> GELSAYTIVVGTVLTGFGFTTPLGLALIGFGTLIPVLFPAQDQSNTWSDFITQTKNIIKKEIASTYISNANKILNRSFNVISTYHNHLKTWENNPNPQNTQDVRTQIQLVHYHFQNVIPELVNSCPPNPSDCDYYNILVLSSYAQAANLHLTVLNQAVKFEAYLKNNRQFDYLEPLPTAIDYYPVLTKAIEDYTNYCVTTYKKGLNLIKTTPDSNLDGNINWNTYNTYRTKMTTAVLDLVALFPNYDVGKYPIGVQSELTREIYQVLNFEESPYKYYDFQYQEDSLTRRPHLFTWLDSLNFYEKAQTTPNNFFTSHYNMFHYTLDNISQKSSVFGNHNVTDKLKSLGLATNIYIFLLNVISLDNKYLNDYNNISKMDFFITNGTRLLEKELTAGSGQITYDVNKNIFGLPILKRREEQGNPTLFPTYDNYSHILSF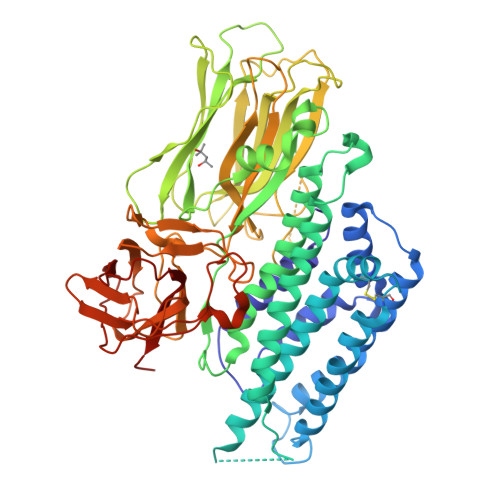IKSLSIPATYKTQVYTFAWTHSSVDPKNTIYTHLTTQIPAVKANSLGTASKVVQGPGHTGGDLIDFKDHFKITCQHSNFQQSYFIRIRYASNGSANTRAVINLSIPGVAELGMALNPTFSGTDYTNLKYKDFQYLEFSNEVKFAPNQNISLVFNRSDVYTNTTVLIDKIEFLPITR> ISEV;> GIEDLISEVAQGALTLSLPKQQDSLPDTKASGPAHSKEVPALTAVETGATNPLAPSDTVQTRHVVQRRSRSESTIESFFARGACVAIIEVDNEQPTTRAQKLFAMWRITYKDTVQLRRKLEFFTYSRFDMEFTFVVTANFTNANNGHALNQVYQIMYIPPGAPTPKSWDDYTWQTSSNPSIFYTYGAAPARISVPYVGLANAYSHFYDGFAKVPLKTDANDQIGDSLYSAMTVDDFGVLAVRVVNDHNPTKVTSKVRIYMKPKHVRVWCPRPPRAVPYYGPGVDYRNNLDPLSEKGLTTY;> SPNVEACGYSDRVLQLTLGNSTITTQEAANSVVAYGRWPEFIRDD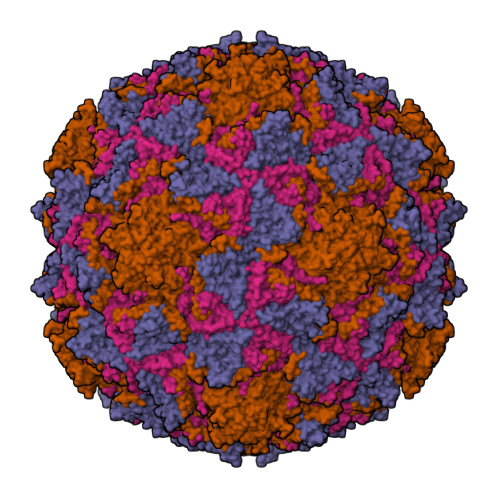EANPVDQPTEPDVATCRFYTLDTVMWGKESKGWWWKLPDALRDMGLFGQNMYYHYLGRSGYTVHVQCNASKFHQGALGVFAIPEYCLAGDSDKQRYTSYANANPGERGGKFYSQFNKDNAVTSPKREFCPVDYLLGCGVLLGNAFVYPHQIINLRTNNSATIVLPYVNALAIDSMVKHNNWGIAILPLSPLDFAQDSSVEIPITVTIAPMCSEFNGLRNVTAPKFQ;> GLPVLNTPGSNQYLTSDNHQSPCAIPEFDVTPPIDIPGEVKNMMELAEIDTMIPLNLESTKRNTMDMYRVTLSDSADLSQPILCLSLSPAFDPRLSHTMLGEVLNYYTHWAGSLKFTFLFCGSMMATGKILVAYAPPGAQPPTSRKEAMLGTHVIWDLGLQSSCTMVVPWISNVTYRQTTQDSFTEGGYISMFYQTRIVVPLSTPKSMSMLGFVSACNDFSVRLLRDTTHISQSA;> GAQVSSQKVGAHENSNRAYGGSTINYTTINYYKDSASNAASKQDYSQDPSKFTEPLKDVLIKTAPALN> GPLGSMENVGRLITPAKKLEDTIRLAELVIEVLQQNEEHHAEAFAWWSDLMVEHAETFLSLFAVDMDAALEVQPPDTWDSFPLFQLLNDFLRTDYNLCNGKFHKHLQDLFAPLVVRYVDLMESSIAQSIHRGFERESWEPVNNGSGTSEDLFWKLDALQTFIRDLHWPEE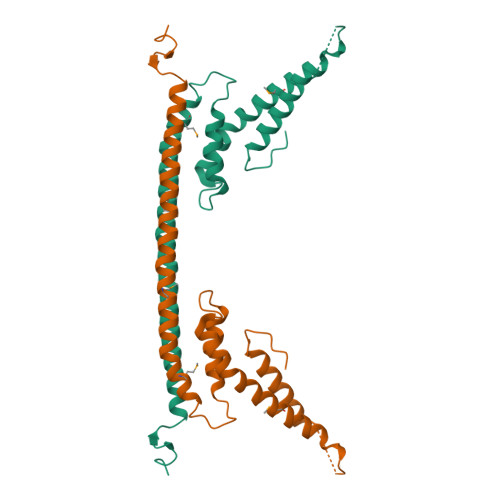EFGKHLEQRLKLMA>MTIKVGINGFGRIGRMVFQALCDDGLLGNEIDVVAVVDMNTDARYFAYQMKYDSVHGKFKHSVSTTKSKPSVAKDDTLVVNGHRILCVKAQRNPADLPWGKLGVEYVIESTGLFTVKSAAEGHLRGGARKVVISAPASGGAKTFVMGVNHNNYNPREQHVVSNASCTTNCLAPLVHVLVKEGFGISTGLMTTVHSYTATQKTVDGVSVKDWRGGRAAALNIIPSTTGAAKAVGMVIPSTQGKLTGMAFRVPTADVSVVDLTFIATRDTSIKEIDAALKR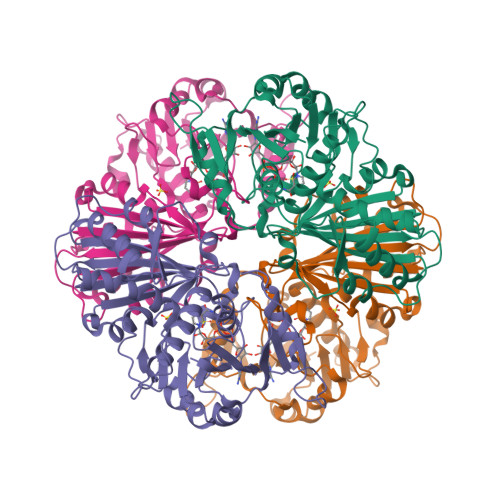ASKTYMKNILGYTDEELVSADFISDSRSSIYDSKATLQNNLPNERRFFKIVSWYDNEWGYSHRVVDLVRHMAARDRAAKL[6x]>[3x]VRKATAAEIAALPRQKVELVDPPFVHAHSQVAEGGPKVVEFTMVIEEKKIVIDDAGTEVHAMAFNGTVPGPLMVVHQDDYLELTLINPETNTLMHNIDFHAATGALGGGGLTEINPGEKTILRFKATKPGVFVYHCAPPGMVPWHVVSGGNGAIMVLPREGLHDGKGKALTYDKIYYVGEQDFYVPRDENGKYKKYEAPGDAYED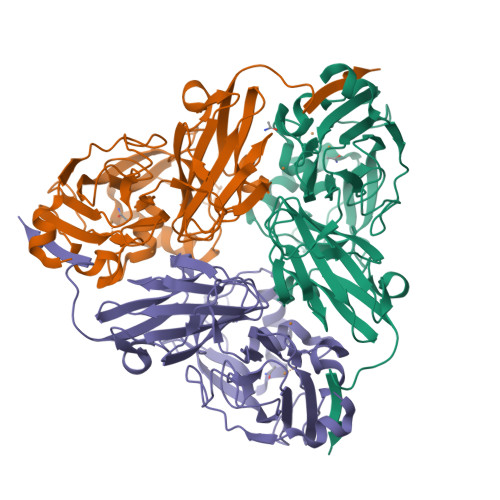TVKVMRTLTPTHVVFNGAVGALTGDKAMTAAVGEKVLIVHSQANRDTRPHLIGGHGDYVWATGKFNTPPDVDQETWFIPGGAAGAAFYTFQQPGIYAYVNHNLIEAFELGAAAHFKVTGEWNDDLMTSVLAPSGT>TLHNIITDTENVQGSFSKHEFQAETKKLLDIVARSLYSEKEVFIRELISNGSDALEKLRHRMITAGGDTAPMEIHLQTDSVKGTFTIQDTGVGMNKEDLVSNLGTIARSGSKAFLDALQNQAEASSSIIGQFGVGFYSAFMVADKVEVYSQSAEADAPGYKWSSDGSGVFEVAEASGVRQGTKIVLHLKDDCKEFSSEDRVKEVVTKYSNFVSFPIFLNGRRLNTLQALWMMEPKDISEWQHEEFYRYVAQAYDKPRYTLHYRADAPLNIRSIFYVPEMKPSMFDVSREMGSSVALYSRKILIQTKATDILPKWLRFLRGVVDSEDIPLNLSRELLQESALIRKLRDVLQQRVIRFLLDQSKKDPEKYARFFEDYGLFMREGIVTTGEQSVKEDIAKLLRFESSALPAGQQTSLMEYSSRMKAGTRNIYYLCAPNRHLAEHSPYFEAMKQKDMEVLFCFEQFDELTLLHLREFDRKKLISAETDIVVDHYKEEKFQDSKPASERLSSEQAEDLLAWMRNALVQRVT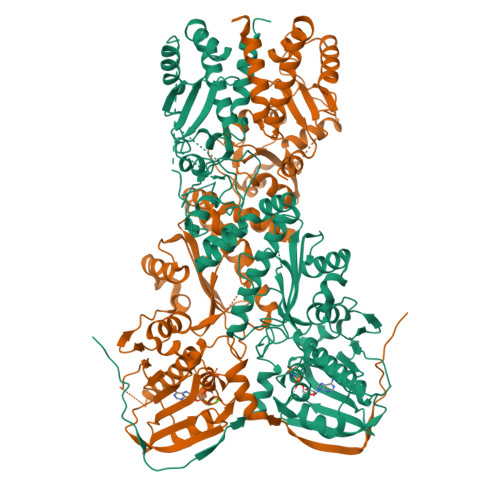NIKVTPRLDTHPAMITVLEMGAARHFLRTQQLARSSEERAQILQPTLEINTGHDLIKKLHALKDSNPELAQLLLEQIYDNAMIAAGLNEDPRPMISRLNQLLTRALEKH[2x]Para-hydroxybenzoate hydroxylase (PHBH) is a group A flavoprotein monooxygenase that hydroxylates p-hydroxybenzoate to protocatechuate (PCA). Among proteins in this clade, Xylophilus ampelinus PobA (XaPobA) preferred PCA as a substrate and is the first known natural PCA 5-hydroxylase (PCAH). The overall structure of XaPobA comprised a homodimer, with each unit binding an oxidized form of FAD in its active site. The XaPobA monomer consisted of FAD-(amino acids 1–73, 88–198, and 267–391)- and substrate (amino acids 74–87 and 199–266)- binding domains.

To understand the substrate recognition mechanism of XaPobA, we determined the PCA-bound structure (XaPobA + PCA) at a resolution of 1.65 Å by growing crystals under imidazole-free conditions and soaking them with PCA. The β-sheets 14 to 16 in the substrate binding domain were located significantly closer to the catalytic center in XaPobA + PCA compared with XaPobA + imidazole, indicating that bound PCA induced XaPobA to adopt a closed conformation. The PCA molecule in the active site was adjacent to the isoalloxazine ring of FAD with the aromatic C5 atom to be hydroxylated facing the ring. The carboxy group of PCA in the XaPobA + PCA structure hydrogen-bonded with the side chain hydroxy groups of Ser212 and Tyr222. The side chain of Arg214 had two alternative conformations, one of which formed a salt bridge with the carboxy group of PCA. In addition to PCA in the active site, we also identified the electron density of an apparently catalytically inert second PCA molecule located near the ribityl moiety of FAD at ∼6 Å from the isoalloxazine ring. The Corey-Pauling-Koltun (CPK) model of the XaPobA + PCA structure showed that the side chains of eight amino acid residues formed a hydrophobic cavity with the aromatic ring of PCA. This was buried with the 3-hydroxy group of PCA enclosed by the Met72, Ile75, Val199, and Trp201 residues and faced the bottom of the cavity. The carbonyl group in the main chain of Thr294 formed a hydrogen bond with the 4-hydroxyl group of PCA and was the only hydrophilic interaction in the cavity. The side chains of Val47 and Ala296 formed a cavity wall parallel to the aromatic ring of PCA, and it was sandwiched between another cavity wall formed by Met210 at the opposite plane of the aromatic ring.

>[2x]MQLSHHHHHHSSGLVPRGSHMRTQVGIVGAGPAGLMLAHLLRREGIDAVVIERAAREHVRTRLRAGVLEQGTVEMLREAGVGGRIDAVGMEMHAIDFRFGGRSHRLDFHEASGGRRAWVYPQHEVVTDLMSACDAGDVPILYEAPVERIEGLEDDRARIVFGQDGAAGEITCDFVAGCDGFRGVSRGSMPAGIARGYDRIYPFGWLGILADAPPASPDVTWGCSDRGFAMMSMRSPTVTRLYLQCEPDEDPDAWSDDRIWSELHRRLDVEGMPSLREGPIRDKGVTAMRSFLSEPMQHGRLFLAGDAAHIVPPTGAKGLNSAMADIKVLAAALVDHYRHGRSDRLATYSERCLRRMWLVQRFSAALCTMVHQFPGQNEFVRRLQRADLDYMTGTHAGRLQFAENFTGLPIE2-cyclopropyl-N-[(2R)-3-hydroxy-3-methylbutan-2-yl]-5H-pyrrolo[2,3-b]pyrazine-7-carboxamide 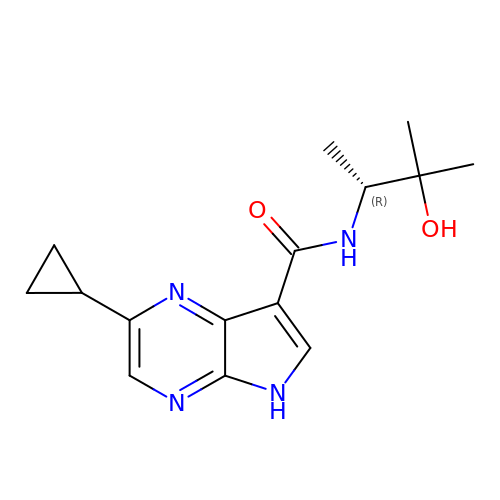| C15 H20 N4 O2 | ODYYFDDUIDLRBK-MRVPVSSYSA-N>MAHHHHHHGICSSAPTLGEIWKRKLNQLDAKEFMAYRRRFVVEVDRNEAREALAKGKTNTGHAVSRGTAKLAWIDERGGVELKGTVVDLGCGRGSWSYYAASQPNVREVKAYTLGTSGHEKPRLVETFGWNLITFKSKVDVTKMEPFQADTVLCDIGESNPTAAVEASRTLTVLNVISRWLEYNQGCGFCVKVLNPYSCDVLEALMKMQARFGGGLIRVPLSRNSTHEMYFVSGIKNNIMGNVTAVSRQLLKRMEEQGGERVVPDYKF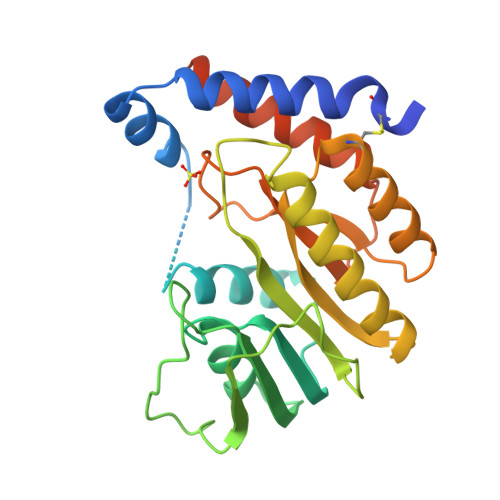STGTRSNL[2x]> CGIVGAIAQRDVAEILLEGLRRLEYRGYDSAGLAVVDAEGHMTRLRRLGKVQMLAQAAEEHPLHGGTGIAHTRWATHGEPSEVNAHPHVSEHIVVVHNGIIENHEPLREELKARGYTFVSETDTEVIAHLVNWELKQGGTLREAVLRAIPQLRGAYGTVIMDSRHPDTLLAARSGSPLVIGLGMGENFIASDQLALLPVTRRFIFLEEGDIAEITRRSVNIFDKTGAEVKRQDIESNLQYDAGDKGIYRHYMQKEIYEQPNAIKNTLTGRISHGQVDLSELGPNADELL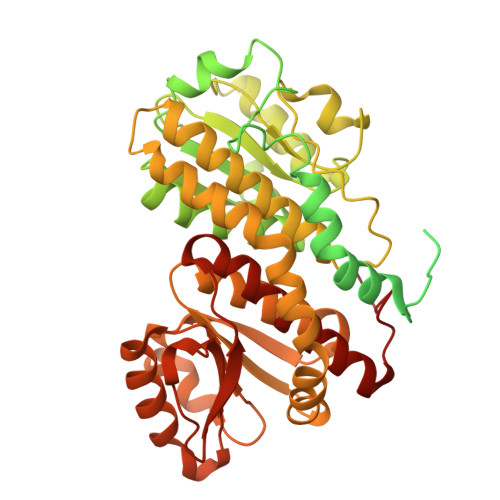SKVEHIQILACGTSYNSGMVSRYWFESLAGIPCDVEIASEFRYRKSAVRRNSLMITLSQSGETADTLAGLRLSKELGYLGSLAICNVPGSSLVRESDLALMTNAGTEIGVASTKAFTTQLTVLLMLVAKLSRLKGLDASIEHDIVHGLQALPSRIEQMLSQDKRIEALAEDFSDKHHALFLGRGDQYPIALEGALKLKEISYIHAEAYAAGELKHGPLALIDADMPVIVVAPNNELLEKLKSNIEEVRARGGQLYVFADQDAGFVSSDNMHIIEMPHVEEVIAPIFYTVPLQLLAYHVALIKGTDVDQPRNLAKSVTVE> MRSRRVDVM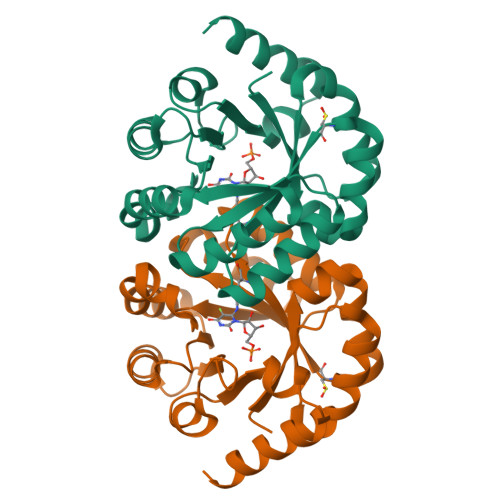DVMNRLILAMDLMNRDDALRVTGEVREYIDTVKIGYPLVLSEGMDIIAEFRKRFGCRIIADFKVADIPETNEKICRATFKAGADAIIVHGFPGADSVRACLNVAEEMGREVFLLTEMSHPGAEMFIQGAADEIARMGVDLGVKNYVGPSTRPERLSRLREIIGQDSFLISPGVGAQGGDPGETLRFADAIIVGRSIYLADNPAAAAAGIIESIKDLLIPEDPAANKARKEAELAAATA2,3-DIFLUOROBENZYL ALCOHOL 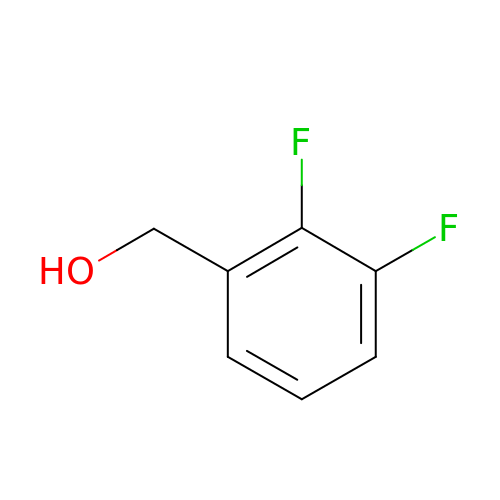| C7 H6 F2 O | JSFGDUIJQWWBGY-UHFFFAOYSA-N>[2x]MGSSHHHHHSSGLVPRGSHMQMIAEIYYERGTIVVKGDAHVPHAKFDSRSGTYRALAFRYRDIIEYFESNGIEFVDNAADPIPTPYFDAEISLRDYQEKALERWLVDKRGCIVLPTGSGKTHVAMAAINELSTPTLIVVPTLALAEQWKERLGIFGEEYVGEFSGRIKELKPLTVSTYDSAYVNAEKLGNRFMLLIFDEVHHLPAESYVQIAQMSIAPFRLGLTATFEREDGRHEILKEVVGGKVFELFPDSLAGKHLAKYTIKRIFVPLAEDERVEYEKREKVYKQFLRARGITLRRAEDFNKIVMASGYDERAYEALRAWEEARRIAFNSKNKIRKLREILERHRKDKIIIFTRHNELVYRISKVFLIPAITHR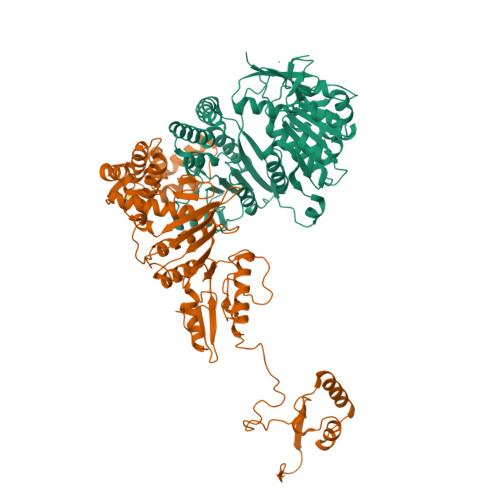TSREEREEILEGFRTGRFRAIVSSQVLDEGIDVPDANVGVIMSGSGSAREYIQRLGRILRPSKGKKEAVLYELISRGTGEVNTARRRKNAAKGAA;>MLPKELLDVRRAKGRIFPKFADERDYELAEKVIEIFKKGLGKKYGNLMKQARKLENAKNFKKVRGFIRVLENHCIEKSCAFDVDSELEPRKVRMLLFEHGFVTSKKERDRVLEYVARYFSTTPETVERAMYADREEELILTKFRPLTPDNLIKLYNLSLLQTTLFNALRLTFWASDRHKEIFRSIKRLGLMYELYEDSGRLMVEVTGAATLLKMTRKYGVSFAKLIPWILRAKNWFIRAEISDFDRLYIMEIDDRIRDLFPDVEERLSYDSTLEEEFARKMQMLGYEVEREPDVVKAGKYAFIPDFAVNLGDKKVYIEIAGFWTDEYLRKKAEKIKSSSIPLILIAREDFGDGGANVKDVILFSRKIPYGEVIKALKRYKPEKKVEGDVVELENFAEVPSEYVIAGKYAVRREIFEEIKREIEVSNPSTLEDIKAILKKYGLGESAIRAFGYRVRWIGLGEAVIERTD[2x]>[3x]MKKYTCKICGYIYNPEDGDPDNGVNP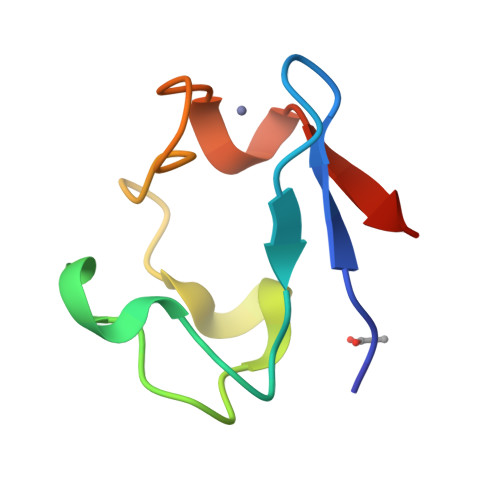GTDFKDIPDDWVCPICGAPKSEFEEVEE N-[2-chloro-5-(trifluoromethyl)phenyl]-2-[1-(4-methoxyphenyl)-4-oxo-1,4-dihydro-5H-pyrazolo[3,4-d]pyrimidin-5-yl]acetamide | C21 H15 Cl F3 N5 O3 | 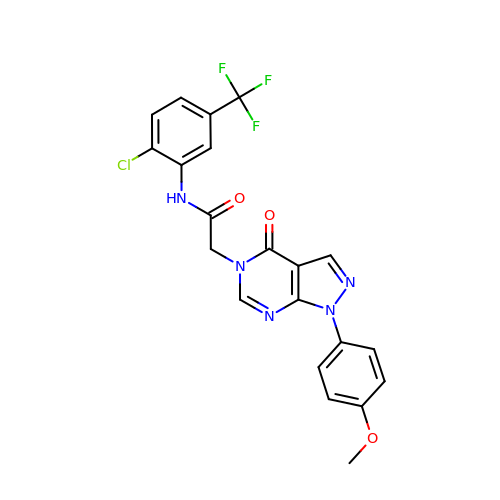VVMPLFOVCSRJQQ-UHFFFAOYSA-N> SNAMQAIRSILVVIEPDQLEGLALKRAQLIAGVTQSHLHLLVCEKRRDHSAALNDLAQELREEGYSVSTNQAWKDSLHQTIIAEQQAEGCGLIIKQHFPDNPLKKAILTPDDWKLLRFAPCPVLMTKTARPWTGGK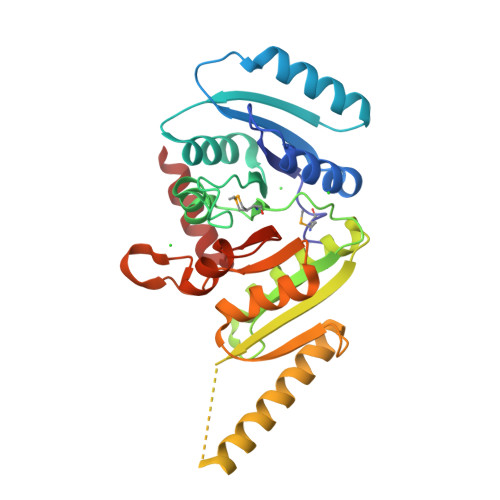ILAAVDVGNNDGEHRSLHAGIISHAYDIAGLAKATLHVISAHPSPMLSSADPTFQLSETIEARYREACRTFQAEYGFSDEQLHIEEGPADVLIPRTAQKLDAVVTVIGTVARTGLSGALIGNTAEVVLDTLESDVLVLKPDDIIAHLEELASKE>GSLDGPYQSTSFKPPSDYWILLNPTNQQVVLEGTNKTDIWVALLLVEPNVTNQSRQYTLFGETKQITVENNTNKWKFFEMFRSSVSAEFQHKRTLTSDTKLAGFLKHYNSVWTFHGETPHATTDYSSTSNLSEVETTIHVEFYIIPRSQESKCVEYINTGL[2x]

RV is a non-enveloped double-stranded RNA (dsRNA) virus with three concentric capsid layers encapsidating eleven dsRNA segments. The outermost layer contains the glycoprotein VP7 and the protease-sensitive spike protein VP4, which define the classification of RVs into G and P genotypes, respectively. RVs use the VP8* domain of the spike protein VP4 to recognize specific host glycans in a genotype-dependent manner. Our studies show that VP8* of these genotypes engages the type I precursor glycan (Galβ1,3-GlcNAc) at a unique and conserved binding site that is present in all P, P and P HRVs, and the subtle sequence and structural changes lead to an altered glycan configuration at the reducing end in the neonate-specific P RV, that may play a key role in the age-restricted tropism of some P strains.

The structure of the neonate-specific P VP8* has not been determined previously. To examine whether the VP8* structure of P differs from that of other HRV genotypes including P, P, P, and P, and whether it can bind glycans as observed in P and P, we first determined the crystal structure of VP8* of a neonate-specific P HRV strain RV3 at 2.0 Å resolution. Similar to other VP8* structures, the P VP8* has a β-sandwich galectin fold with a distinct cleft between the two twisted β-sheets. The cleft in the P VP8* is noticeably wider compared to that observed in the VP8* of P HRV, but similar to that observed in the VP8* of other HRV genotypes including P, P, and P. Comparative analysis with the glycan bound structures of P and P VP8*s shows how sequence variations in the P VP8* leads to the loss of A-type HBGA binding observed with P VP8* and how interaction with type I glycans in P VP8* is unlikely to be similar to that observed in P VP8*. The sidechain of R101 in P, which makes a strong hydrogen bond interaction through its side chain with A-type HBGA, is substituted by isoleucine in P which cannot make such an interaction; the hydrophobic residue Y188, which is crucial for stabilizing A-type glycan in P VP8*, is replaced by a hydrophilic amino acid D186 in the P VP8*. The residue R187 involved in direct hydrogen bonds with Gal of LNT in P VP8* is replaced by T184 in P VP8*. The residues Y156 and W178, which provide hydrophobic interaction with LNT in P VP8*, are changed to T156 and H177, respectively. The J-K loop that interacts with LNT in P VP8* projects away in the P[6]VP8* structure. These observations indicate that the neonate-specific P VP8* cannot bind LNT at the same site as P VP8* and likely has a distinct site for type I glycan binding.BIPHENYL | 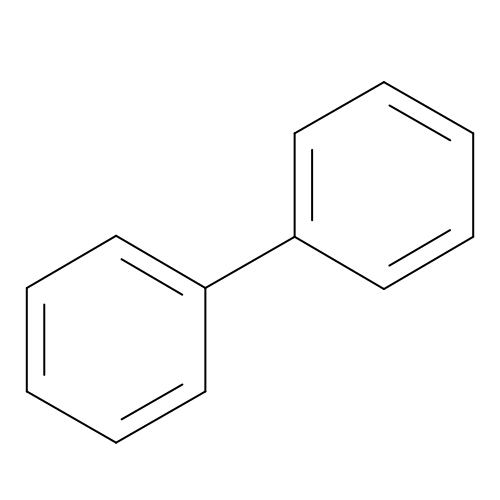C12 H10 | ZUOUZKKEUPVFJK-UHFFFAOYSA-N> MIYLRKANERGHANHGWLDSWHTFSFANYYDPNFMGFSALRVINDDVIEAGQGFGTHPHKDMEILTYVLEGTVEHQDSMGNKEQVPAGEFQIMSAGTGIRHSEYNPSSTERLHLYQIWIMPEENGITPRYEQRRFDAVQGKQLVLSPDARDGSLKVHQDMELYRWALLKDEQSVHQIAAERRVWIQVVKGNVTINGVKASTSDGLA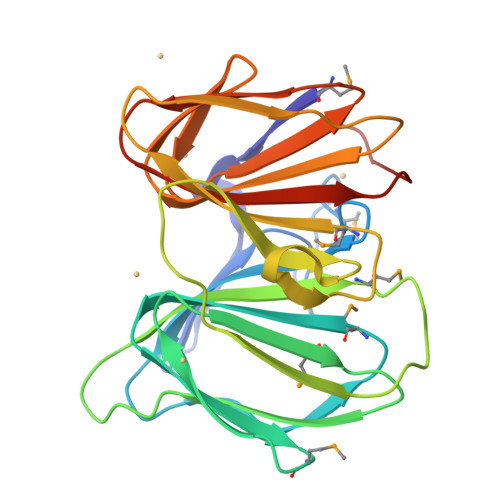IWDEQAISIHADSDSEVLLFDLPPVSGRVEHHHHHH> MDSSTWSPKTTAVTRPVETHELIRNAADISIIVIYFVVVMAVGLWAMFSTNRGTVGGFFLAGRSMVWWPIGASLFASNIGSGHFVGLAGTGAASGIAIGGFEWNALVLVVVLGWLFVPIYIKAGVVTMPEYLRKRFGGQRIQVYLSLLSLLLYIFTKISADIFSGAIFINLALGLNLYLAIFLLLAITALYTITGGLAAVIYTDTLQTVIMLVGSLILTGFAFHEVGGYDAFMEKYMKAIPTIVSDGNTTFQEKCYTPRADSFHIFRDPLTGDLPWPGFIFGMSILTLWYWCTDQVIVQRCLSAKNMSHVKGGCILCGYLKLMPMFIMVMPGMISRILYTEKIACVVPSECEKYCGTKVGCTNIAYPTLVVELMPNGLRGLMLSVMLASLMSSLTSIFNSASTLFTMDIYAKVRKRASEKELMIAGRLFILVLIGISIAWVPIVQSAQSGQLFDYIQSITSYLGPPIAAVFLLAIFWKRVNEPGAFWGLILGLLIGISRMITEFAYGTGSCMEPSNCPTIICGVHYLYFAIILFAISFIT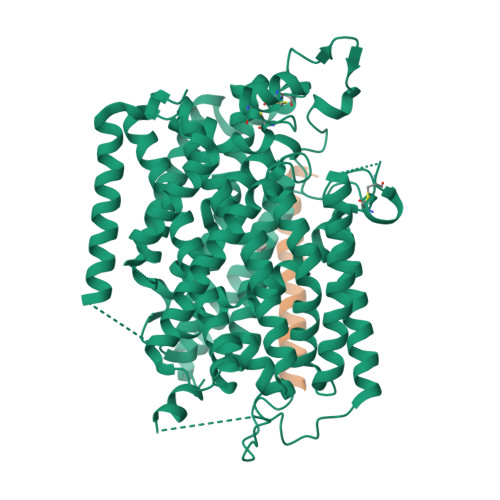IVVISLLTKPIPDVHLYRLCWSLRNSKEERIDLDAEEENIQEGPKETIEIETQVPEKKKGIFRRAYDLFCGLEQHGAPKMTEEEEKAMKMKMTDTSEKPLWRTVLNVNGIILVTVAVFCHAYFA;> MSALSLLILGLLTAVPPASCQQGLGNLQPWMQGLIAVAVFLVLVAIAFAVNHFWCQEEPEPAHMILTVGNKADGVLVGTDGRYSSMAASFRSSEHENAYENVPEEEGKVRSTPM>MTLVPYVVEDTGRGERAMDIYSRLLKDRIVMIGQEITEPLANTVIAQLLFLMSEDPTKDIQIFINSPGGYITAGLAIYDTIRFLGCDVNTYCIGQAASMGALLLSAGTKGKRYALPHSRMMIHQPSGGIIGTSADIQLQAAEILTLKKHLSNILAECTGQSVEKIIEDSERDFFMGAEEAIAYGLIDKVISSAKETKDKSIAS[14x]

Caseinolytic proteases (Clp) are a family of conserved multiple-subunit enzymes found in bacteria and higher organisms that have become an attractive and novel therapeutic target to combat infection. ClpP assembles into tetradecameric barrels consisting of two heptameric rings. These barrels interact with hexameric AAA+ unfoldases, such as ClpX, ClpA, or ClpC, to unfold the targeted protein and facilitate its entrance into the proteolytic barrel. Proteolytic activity requires alignment of the catalytic triad through conformational changes of the handle domain that composes the interface between heptamer rings.

Here, we report the first crystal structure of full-length ClpP2 as an inactive homotetradecamer in a complex with a candidate antibiotic at 2.66 Å resolution. The asymmetric unit of ctClpP2 includes two opposing heptameric rings that form a tetradecamer with a height of 77 Å and a diameter of 95 Å. The monomers in the crystal structure follow the canonical ClpP fold with the secondary structure consisting of a set of aligned α-helices (α2- α5) behind four β-sheet motifs aligned in the direction of the α-helices (β1-β3 and β5). Lack of hydrogen bonding among the triad indicates that the ctClpP2 residues are in an inactive form and that a conformational change is required for the catalytic residues to interact. First, ctClpP2 is the only ClpP among those compared that has both a flexible N terminus and a mini-helix, also called α8, at the C terminus. Second, the handle loop is more compact and the α5 helix that follows is 2∼3 helical turns shorter in ctClpP2. This means oligomerization leads to a ctClpP2 tetradecamer that is shorter in height, 77 Å, compared to counterparts from other species, > 85 Å, except for saClpP that also has a compact handle domain. The C-terminal loop of ctClpP2 that includes a mini-helix, α8, is situated such that it acts like a lid toward the hydrophobic pocket and mediates a neighboring positive electrostatic environment with residues Lys197 and Lys199 in addition to residues Arg28 and Lys58. For ctClpP2 and ecClpP, the hydrophobic pocket is proximal to a cluster of positively charged surfaces that interact with the electron-rich fluorines of the trifluoromethylpyridine group. While activation of ctClpP2 would have been expected when analyzing drug-bound crystal structures of ClpP homologs, we observed a misaligned triad and thus the inactive form of ctClpP2.>[2x]MAHHHHHHMQIEGCVACVTGADRGLGAGLLEALLERGARKVYAGVRKKECLSDVGPRVVPVEIDITNVEQVARAASRAKDITLLINNAG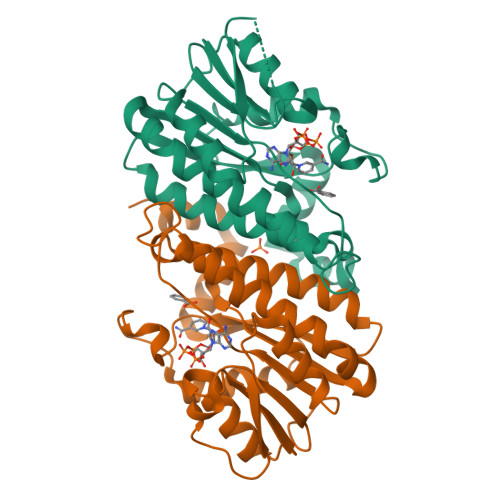LNRMQPVLEAHDPEAARAEMEVNYFGTLNMMRAFSPALKSNGGAIINVLSILARVALPSMASLSASKAAALRMTEGARAELAPHRVRVISVLPGPIDTEMSRNVPPPKIAVREAVDAVLAALEGGADEVYMGAMAQEIAQGLAADRQALHARLLTP> MSLLKNYPPSYLYPFRHPK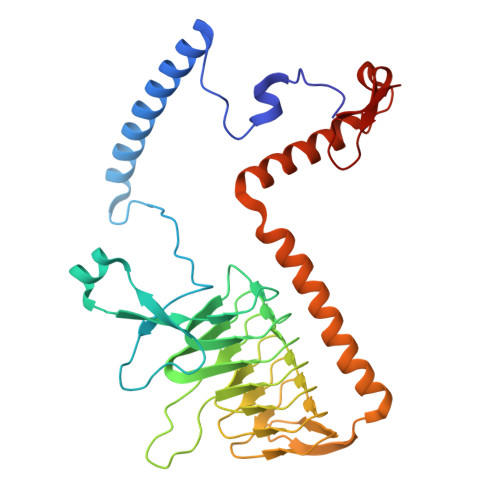PEGVIEKVLFNLGSLFRSAGQGMDELGSLMLGNGGMQESVGPNLAYAPVKYNPAAAPKAGIVAPIPASAQRVLGVKEIVLPSKAESTFIAPNANVLGDVKIGAKSSIWYGAVLRGDVNSIEIGDNTNVQDNVTIHVAKHSIDGKLRNTVIGNNVTIGHCATIHACTIADNVIIGMGATVLDGVKVESGSIVGAGSIVPPNTVIPAGQVWVGNPAKFIRNVLPEENGFIASSANNYDLLGQQHKFENSKVFEEMLVEEEIAKDRELLEDKNLAVHQLYIFDPQTQLAARPRR>QKEYMEYRPLGEEIERIRKGKNIPLRVFDENGVSSRSYQRFVQGNSELRISDLAIIVEILSISPMEMTEKLTPMSKTVLAKEQFNQAIF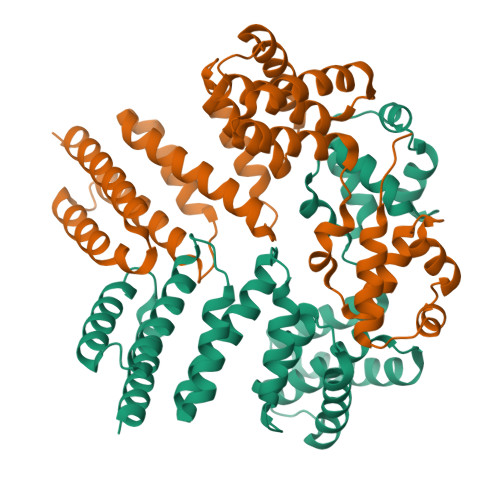SKNFQESSRIVADYRAYYEKSSFALGKQEVMYSMLALEYLFNPQTVVTKEEIIALENQILERLINADVYTIFNLKFLALQKNVGLQPFPTSLLFRVLQSVNEREIIDIRSLEIIEQVIIDFLFAAIVSQNVPHILHVLSMFKEYEVGENNWRMILWKKIAEKIEMILTNEEIFADWSIFKEQILLSITLFLPKAKQEFFAGQLEKIEDSLKEIKENG[2x]>[8x]AEITLISHKTLGSQLRDGMKLATGRIACREPHDGFHIWINASQNGKVGHYIVQNNRETKHELKVKIGGGGWSSSLIEGQRGVYRQGEEKQAI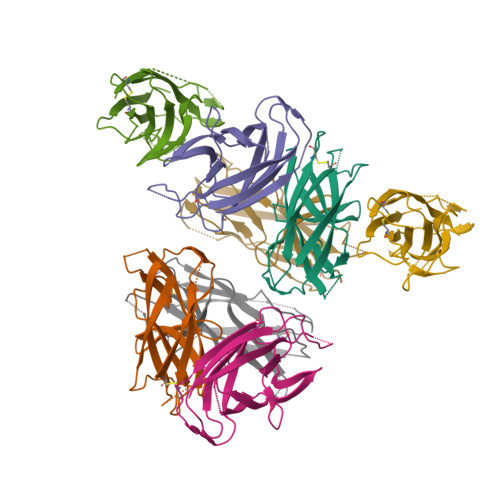FDIMSDGNQYSAPGEYIFSVSGECLISRGDNKQALERPPIKATETIRLTV>[6x]SMSSLDINEQRALIKSAHRYI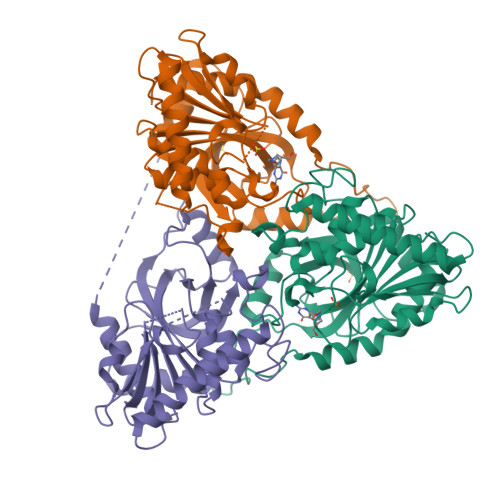SEKLEDHFSSEFLPKALVICGEGLSGISTKIADEPKPLILSYSTIPGFKVSTVPGHSGELIFGYMNGAPVVLMNGRLRSYEGHSLAETVHPIRALHLLGSINVLIVTNAAGGINASFKAGDLMCVYDHINFPGLCGFHPLRGANFDEFGPRFLATSDAYDLELRKLLFSKKKELNIERKIHEGTYSYVHGPTFESRAESRFLRLAGTDAVGMSTVPEVVTARHCGWRVLALSLITNECVVDPPASAHDENPVPIQEGKATHEEVLENSAKASKDVQELIFSVVAEI> MGHHHHHHAQLYACQDPTIFEERHLKYISQLGKGNFGSVELCRYDPLGDNTGALVAVKQLQHSGPDQQRDFQREIQILKALHSDFIVKYRGVSYGPGRQSLRLVMEYLPSGCLRDFLQRHRARLDASRLLLYSSQICKGMEYLGSRRCVHRDLAARNILVESEAHVKIADFGLA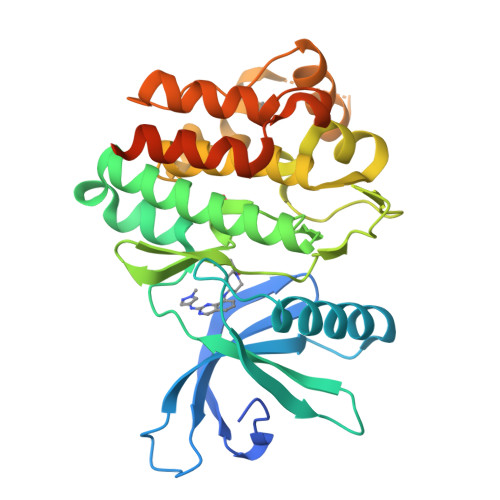KLLPLDKDYYVVREPGQSPIFWYAPESLSDNIFSRQSDVWSFGVVLYELFTYCDKSCSPSAEFLRMMGSERDVPALSRLLELLEEGQRLPAPPACPAEVHELMKLCWAPSPQDRPSFSALGPQLDMLWSGSRGCETHAFTAHPEGKHHSLSFS> GIGTGFPFDPHYVEVLGERMHYVDVGPRDGTPVLFLHGNPTSSYVWRNIIPHVAPTHRCIAPDLIGMGKSDKPDLGYFFDDHVRFMDAFIEALGLEEVVLVIHDWGSALGFHWAKRNPERVKGIAFMEFIRPIPTWDEWPEFARETFQAFRTTDVGRKLIIDQNVFIEGTLLMGVVRPLTEVEMDHYREPFLNPVDREPLWRFPNELPIAGEPANIVALVEEYMDWLHQSPVPKLLFWGTPGVLIPPAEAARLAKSLPNCKAVDIGPGLNLL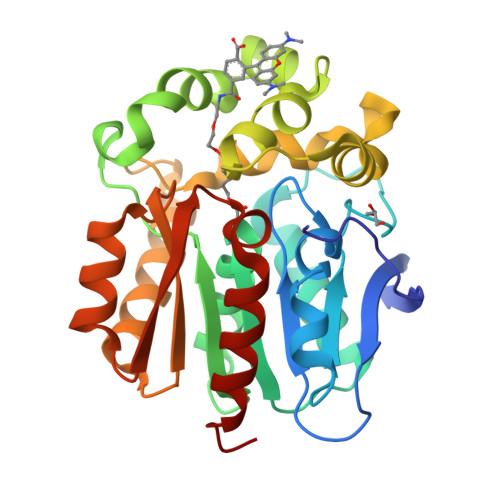QEDNPDLIGSEIARWLSTLEI>[2x]MTPEAIIEDRRFQETLDKIRKEEGYDFAAIAFYESNKPSSPIKWHYVSGNKNNRFKLIILRKGRGLA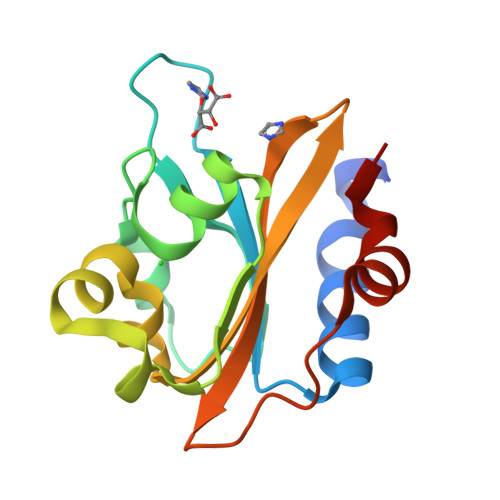GTVMKTGKRMVIANVGLALGPEEKIDAPILLSESLTAVLAVPLWYKNQVYGVLLFGQRDGRPLPKIFDNDDIQRKFGIFNDDK> C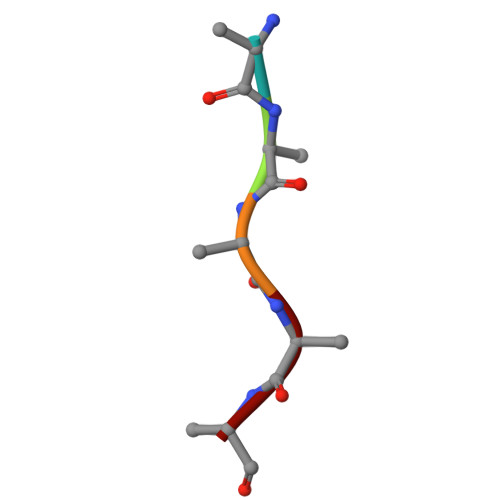YRKL>[4x]MSLSRFAKGLVQGARTSVGLAIPDLTNPYFPAFASSVVELATLRGWHVVVDDYGHGGRSGLDAVEHLAPQVDAVIGYLGGYADQAQTVLGRRP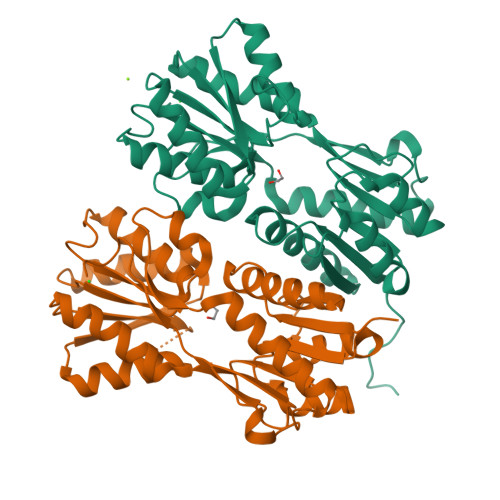LIVLDENPGGAAGSINFDYQHAAKVAVAQLMDSKRQHIAYLEAGSASESDEPVPCTVRGKAVAGRLDELGASWSLIVAEETAEAAREAAAAFLREHPETDGILAFNDLMAAGVLKALSGSGRRVPEDCAVIGMDGIPLGELLSPQLSTMALDLREVGRAAVELLVGLLSGAVTPGSQSSRTTLKHRLVLRESTEGHHHHHH> MTTKNTLQPTEAAYIAGFLDGDGSIYAKLIPRPDYKDIKYQVSLAISFIQRKDKFPYLQDIYDQLGKRGNLRKDRGDGIADYTIIGSTHLSIILPDLVPYLRIKKKQANRILHIINLYPQAQKNPSKFLD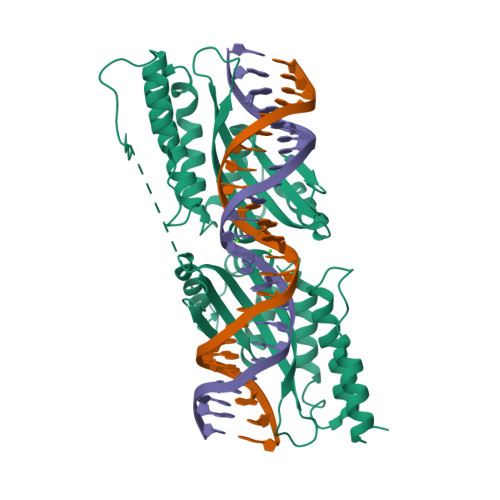LVKIVDDVQNLNKRADELKSTNYDRLLEEFLKAGKIESSPTGSGSGSKHPTLTLPTTTSQENLPNGSGSGSGTMTTKNTLQPTEAAYIAGFLDGDGSIYAKLIPRPDYKDIKYQVSLAISFIQRKDKFPYLQDIYDQLGKRGNLRKDRGDGIADYTIIGSTHLSIILPDLVPYLRIKKKQANRILHIINLYPQAQKNPSKFLDLVKIVDDVQNLNKRADELKSTNYDRLLEEFLKAGKIESSP> GSSIAERSVPIAVPVPTGGDDPTKIAMLGLTFDDVLLLPAASDVLPANADTSSQLTKKIRLKVPLVSSAMDTVTEARMAIAMARAGGMGVLHRNLPVAEQAAQVETVKRSGGLLVGAAVGVGDDAWERAMALRDAGVDVLVVDTAHAHNRKVLDMVHRLKTTVGDEIEVVGGNVATRAAAAALVEAGADAVKVGVGPGSICTTRVVAGVGAPQITAILEAVAACAPHGVPVIADGGLQYSGDIAKALAAGASTAMLGSLLAGTAESPGELILVNGKQFKSYRGMGSLGAMQGRGGAKSYSKDRYFQDDALSEDKLVPEGIEGRVPFRGPLSTVIHQLVGGLRAAMGYTGSATIEELQQAQFVQITAAGLKESHPHDITMTVEAPNYYAR

IMPDH is an essential enzyme that catalyzes the NAD+-dependent conversion of inosine 5′-monophosphate (IMP) to xanthosine 5′-monophosphate (XMP) in the de novo purine biosynthesis pathway. As the crystal structure of Mycobacterium thermoresistible (Mth) IMPDH (GuaB2) was elucidated during the course of this study, the modes of binding of seven compounds to Mth IMPDH were also analysed by X-ray crystallography and docking analyses performed for three others. Computational analysis of the Mth IMPDH (GuaB2) structure revealed two main hotspot regions, both of which were located within the NAD binding pocket. All compounds were evaluated for structural analysis and co-crystal structures were obtained for seven of these, namely compounds 14, 18, 22, 27, 35, 37 and 45.

Replacement of the cyclohexyl by a cycloheptyl ring (compound 14) reduced both enzyme and whole-cell activities by approximately one order of magnitude (MIC90: 31.2 μM, IC50: 0.83 μM) while maintaining target selectivity. The co-crystal structure of 14 with Mth IMPDH confirmed the binding of this compound to the NAD-binding pocket of IMPDH in a similar manner to compound 1. Pharmacophore analysis of the binding highlighted the pivotal role of interactions with 14 made at both hotspot regions identified. In the first hotspot region, all of the analogues made extensive pi interactions with both IMP and A285 (A269 in the Mth structure). The tails of the enzyme inhibitors extended up into the second hotspot region, where they all made strong pi interactions with the Y487′ (Y471′ in the Mth structure) side chain from the adjacent molecule in the tetramer. The compounds 14, 18, 22, 27, 35, 37 and 45 were also able to make additional interactions to P61′ side chain from the adjacent protomer.>GGGTACCC[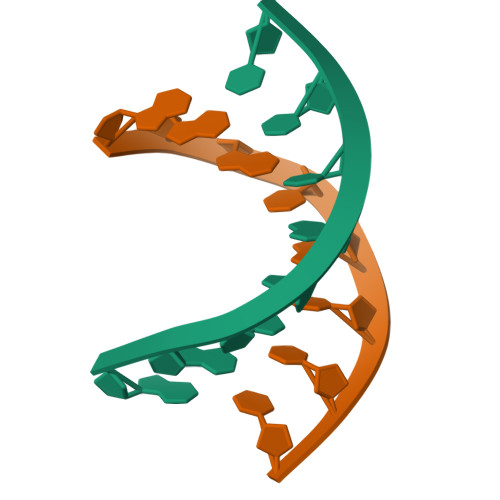2x]>[9x]AQVQQLTPAQQAALRNQQAMAANLQARQIVLQQSYPVIQQVETQTFDPANRSVFDVTPANVGIVKGFLVKVTAAITNNHATEAVALTDFGPANLVQRVIYYDPDNQRHTETSGWHLHFVNTAKQGAPFLSSMVTDSPIKYGDVMNVIDAPATIAAGATGELTMYYWVPLA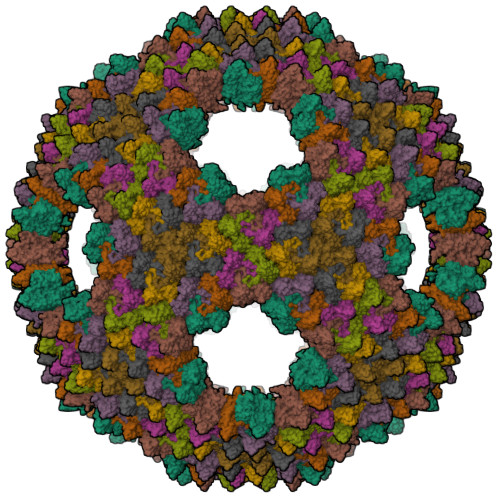YSETDLTGAVLANVPQSKQRLKLEFANNNTAFAAVGANPLEAIYQGAGAADCEFEEISYTVYQSYLDQLPVGQNGYILPLIDLSTLYNLENSAQAGLTPNVDFVVQYANLYRYLSTIAVFDNGGSFNAGTDINYLSQRTANFSDTRKLDPKTWAAQTRRRIATDFPKGVYYCDNRDKPIYTLQYGNVGFVVNPKTVNQNARLLMGYEYFTSRTELVNAGTISTT>[2x]UACUA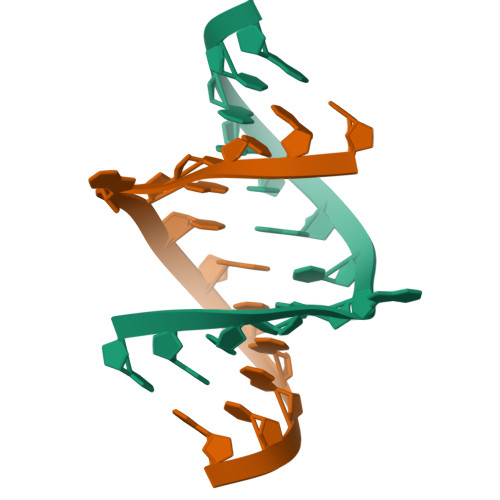ACGUAGUA A key component of the recycling machinery is the endosomal sorting complex for promoting exit 1 (ESCPE-1), which rescues transmembrane proteins from the endolysosomal pathway for transport to the trans-Golgi network and the plasma membrane. The SNX protein family is defined by the presence of a phox-homology (PX) domain that typically binds phosphatidylinositol phospholipids (PtdInsPs), but may also participate in protein–protein interactions. Twelve out of the 33 annotated mammalian SNXs contain an additional carboxy-terminal Bin/Amphiphysin/Rvs (BAR) domain, and are therefore denoted as the PX-BAR or SNX-BAR subfamily. Herein, we show that ESCPE-1 has a single-layer coat organization and suggest how synergistic interactions between ESCPE-1 protomers, phosphoinositides and cargo molecules result in a global arrangement of amphipathic helices to drive tubule formation.

The crystal structure of the SNX1BAR–SNX5BAR complex presented here, together with analytical modeling, revealed that SNX1 comprises a hydrophobic binding hot spot compatible with homodimerization and heterodimerization, whereas SNX5 uses distinct patches of polar residues to preclude homodimerization and enhance heterodimerization. The structure forms an antiparallel dimer of three-helix bundles with a curvature that would fit a circle with a diameter of ~32 nm. The interface buries a large area of 5,114 Å2, of which 78% corresponds to polar surface. SNX1BAR and SNX5BAR exhibit complementary polarity at their distal and proximal interfaces. Consistent with previous predictions, the central region of SNX5BAR has a negative patch, whereas the equivalent region in SNX1BAR is neutral.

>[2x]KMNESDIWFEEKLQEVECEEQRLRKLHAVVETLVNHRKELALNTAQFAKSLAMLGSSEDNTALSRALSQLAEVEEKIEQLHQEQANNDFFLLAELLSDYIRLLAIVRAAFDQRMKTWQRWQDAQATLQKKREAEARLLWANKPDKLQQAKDEILEWESRVTQYERDFERISTVVRKEVIRFEKEKSKDFKNHVIKYLETLLYSQQQLAKYWEAFLPEAKAIS;>[2x]DEVLFTGVKEVDDFFEQEKNFLINYYNRIKDSCVKADKMTRSHKNVADDYIHTAACLHSLALEEPTVIKKYLLKVAELFEKLRKVEGRVSSDEDLKLTELLRYYMLNIEAAKDLLYRRTKALIDYENSNKALDKARLKSKDVKLAEAHQQECCQKFEQLSESAKEELINFKRKRVAAFRKNLIEMSELEIKHARNNVSLLQSCIDLFKNN> MLKVNEFETDTDLRGNINYLFNDEANVVYTYDGTESDLLQNVNEVSKYIEHHMDYQRPRLKVLSDYYEGKTKNLVELTRRKEEYMADNRVAHDYASYISDFINGYFLGNPIQYQDDDKDVLEAIEAFNDLNDVESHNRSLGLDLSIYGKAYELMIRNQDDETRLYKSDAMSTFIIYDNTVERNSIAGVRYLRTKPIDKTDEDEVFTVDLFTSHGVYRYLTNRTNGLKLTPRENSFESHSFERMPITEFSNNERRKGDYEKVITLIDLYDNAESDTANYMSDLNDAMLLIKGNLNLDPVEVRKQKEANVLFLEPTVYVDAEGRETEGSVDGGYIYKQYDVQGTEAYKDRLNSDIHMFTNTPNMKDDNFSGTQSGEAMKYKLFGLEQRTKTKEGLFTKGLRRRAKLLETILKNTRSIDANKDFNTVRYVYNRNLPKSLIEELKAYIDSGGKISQTTLMSLFSFFQDPEL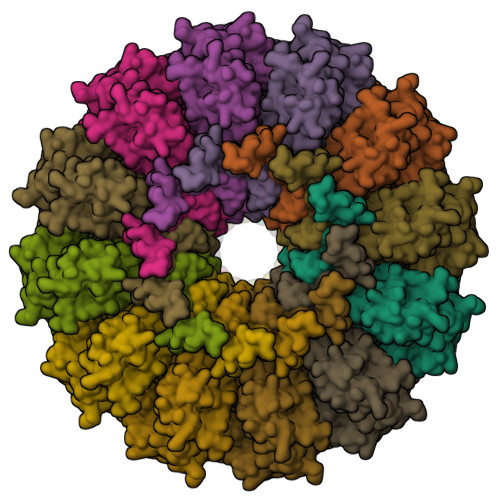EVKKIEEDEKESIKKAQKGIYKDPRDINDDEQDDDTKDTVDKKE;> MTTLADVKKRIGLKDEKQDEQLEEIIKSCESQLLSMLPIEVEQIPERFSYMIKEVAVKRYNRIGAEGMTSEAVDGRSNAYELNDFKEYEAIIDNYFNARTRTKKGRAVFF3-FLUORO-1-(2-HYDROXY-2,2-DIPHOSPHONOETHYL)PYRIDINIUM | C7 H11 F N O7 P2 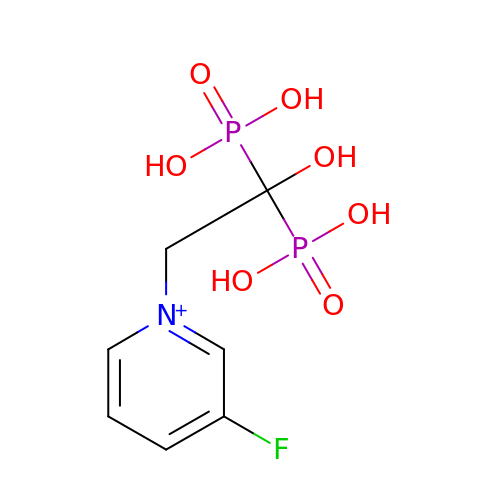| LSEAIOLITUIQJU-UHFFFAOYSA-O> TNL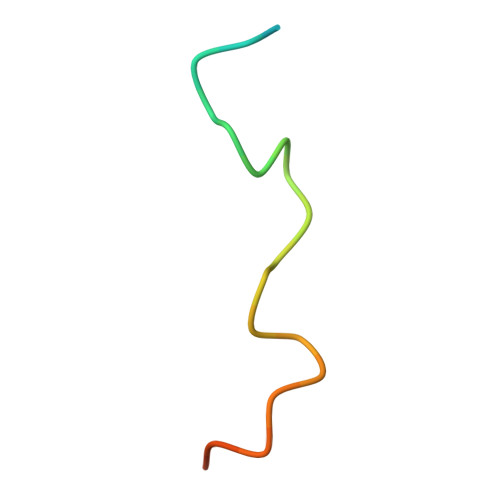DFFQSDPFVGSDPFKDDPFGGAGA>[4x]MNIVVLISGNGSNLQAIIDACKTNKIKGTVRAVFSNKADAFGLERARQAGIATHTLIASAFDSREAYDRELIHEIDMYA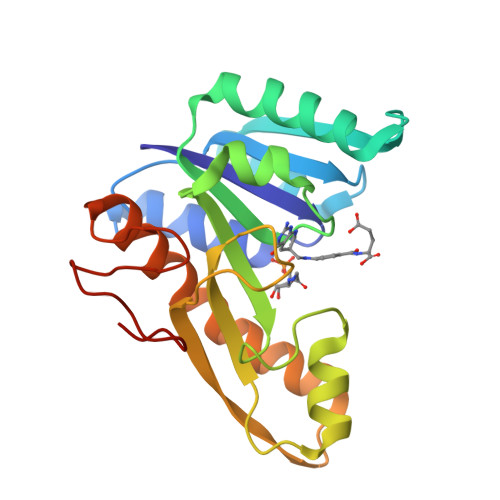PDVVVLAGFMRILSPAFVSHYAGRLLNIHPSLLPKYPGLHTHRQALENGDEEHGTSVHFVTDELDGGPVILQAKVPVFAGDSEDDITARVQTQEHAIYPLVISWFADGRLKMHENAAWLDGQRLPPQGYAADE(1S,2R,3S,4S)-1-{(1S)-2-[(2R,3S,4S)-3,4-dihydroxy-2-(hydroxymethyl)tetrahydrothiophenium-1-yl]-1-hydroxyethyl}-2,3,4,5-tetrahydroxypentyl sulfate | C12 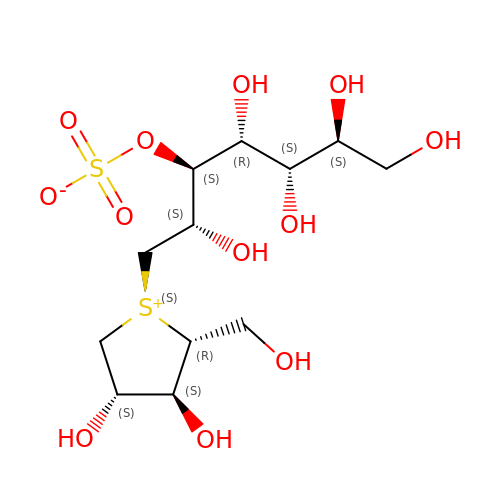H24 O12 S2 | OMKXVFDVAGCPBS-HTOPOKEGSA-N One of the of most well-studied defense collagens is complement component 1q (C1q) found in mammalian serum. A key feature of C1q is its “bouquet” structure, containing six flower-like C-terminal globular domains, an intermediate “branching” collagen-like region, and an N-terminal “stem” where the collagen-like portions bundle together. We have recently recapitulated the unique C1q octadecameric structure in a series of short (∼40 amino acids) synthetic peptides derived from the native sequence of the C1q stem region. Here we use a peptide self-assembly system to design collagenous assemblies based on the C1q collagen-like region.

We next attempted to introduce some asymmetry into our structure by increasing the length of peptide B by including 6 more amino acids at its C-terminus from the full length sequence of C1q30 so it could more easily be identified in the density map. This new peptide we call C1q-B ″carrot-top” peptide (B-Crt). Following this, we were able to use this narrow region model as a starting point to build a model for the full C1q collagenous bundle. The full structure of the C1q cys crt assembly revealed a hollow elongated assembly, ∼ 100 Å long and ∼30–50 Å wide depending on the region of the structure. Top-down views of the map revealed the octadecameric nature of the assembly with six copies of the triple helices. At the N-terminal base of the structure there are spokes extending out of the structure, but these were at too low a resolution to resolve the individual chains. Past the spokes the structure is quite narrow and subsequently widens toward the top as shown in Figure 2c. At the narrowest part the three peptide chains in each PPII trimer are nearly parallel to one another and untwisted. As the structure gets wider toward the C-termini, the peptides wrap around each other with a right-handed twist as expected for a canonical collagen triple helix.

>QLSCTGPPAIPGIPGIPGTPGPDGQPGTPGIKGEKGLPGLAGDH[6x];>[6x]EDLCRAPDGKKGEAGRPGRRGRPGLKGQGEPGAPGIR;>[6x]NTGCYGIPGMPGLPGAPGKDGYDGLPGPKGEPGIP S-[2-({N-[(2R)-2-hydroxy-4-{[(S)-hydroxy(methoxy)phosphoryl]oxy}-3,3-dimethylbutanoyl]-beta-alanyl}amino)ethyl] 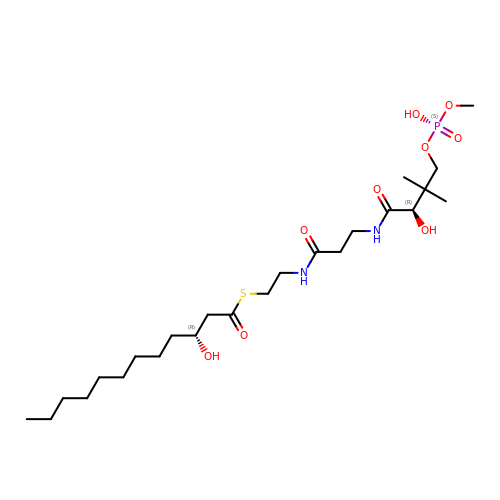(3R)-3-hydroxydodecanethioate | C24 H47 N2 O9 P S | RYLXPSVPJNKBKQ-KNQAVFIVSA-N>[4x]MDWSHPQFEKSNRTPRRFRSRDWFDNPDHIDMTALYLERFMNYGITPEELRSGKPIIGIAQTGSDISPCNRIHLDLVQRVRDGIRDAGGIPMEFPVHPIFENCRRPTAALDRNLSYLGLVETLHGYPIDAVVLTTGCDKTTPAGIMAATTVNIPAIVLSGGPMLDGWHENELVGSGTVIWRSRRKLAAGEITEEEFIDRAASSAPSAGHCNTMGTASTMNAVAEALGLSLTGCAAIPAPYRERGQMAYKTGQRIVDLAYDDVKPLDILTKQAFENAIALVAAAGGSTNAQPHIVAMARHAGVEITADDWRAAYDIPLIVNMQPAGKYLGERFHRAGGAPAVLWELLQQGRLHGDVLTVTGKTMSENLQGRETSDREVIFPYHEPLAEKAGFLVLKGNLFDFAIMKSSVIGEEFRKRYLSQPGQEGVFEARAIVFDGSDDYHKRINDPALEIDERCILVIRGAGPIGWPGSAEVVNMQPPDHLLKKGIMSLPTLGDGRQSGTADSPSILNASPESAIGGGLSWLRTGDTIRIDLNTGRCDALVDEATIAARKQDGIPAVPATMTPWQEIYRAHASQLDTGGVLEFAVKYQDLAAKLPRHNH

Enzymes belonging to the IlvD/EDD protein family are widely distributed among bacteria, archaea, fungi, and algae and in higher plant species. The family includes dihydroxy acid dehydratases (IlvD, DHADHT, DHAD; EC 4.2.1.9), which are involved in short-chain amino acid biosynthesis and catalyse the dehydration of 2,3-dihydroxy-3-methylbutanoate, and aldonic acid dehydratases, which are involved in the metabolism of hexose and pentose sugars via the Entner-Doudoroff (ED) pathway or a modified ED pathway. Pentonate dehydratases from the IlvD/EDD family participate in the non-phosphorylative oxidation pathways of pentose sugars in which D-xylonate dehydratase (XyDHT) and L-arabinonate dehydratase (ArDHT) catalyse the dehydration of D-xylonate and L-arabinonate, respectively.

D-xylonate dehydratase from Caulobacter crescentus (CcXyDHT) shares 42% sequence identity with RlArDHT, and the crystal structure of CcXyDHT shows that this enzyme has a [2Fe-2S] and a Mg2+ ion in its active site, similar to RlArDHT. The structure contained a tetramer in the asymmetric unit in the space group C2. The enzyme is an α/β protein that consists of two domains: a N-terminal domain (residues Asn3-Leu358) and a C-terminal domain (residues Leu383-His591). Each monomer contains one [2Fe-2S] cluster and a Mg2+ ion. The substrate binding site is located in the cavity between the domains, but the [Fe-S] cluster and the Mg2+ binding site are located entirely in the N-terminal domain. The quaternary structure of CcXyDHT is a homotetramer, similar to the homotetrameric structure of RlArDHT. The formation of the extensive dimer interface in CcXyDHT (and in RlArDHT) is essential for the formation of the active site. Although the residues that participate in the binding of Mg2+ and the [2Fe-2S] cofactor are located in the N-terminal domain of the first monomer, the polypeptide chain from the second monomer covers the active site by extending its N-terminal helix (residues 21–33) into the first monomer. In addition, the C-terminus of the dimeric counterpart protrudes into the active site of the first monomer by placing His591, which forms a salt bridge with Glu463, in the active site. The hexacoordination of the Mg2+ ion resembles a square bipyramid in which Glu92, Asp129, Glu463 and a water (or hydroxide ion) are approximately in the plane and another water molecule (or a hydroxide ion) and carbamylated Lys130 are in the axial positions.> MELKHSISDYTEAEFLEFVKKICRAEGATEEDDNKLVREFERLTEHPDGSDLIYYPRDDREDSPEGIVKEIKEWRAANGKSGFKQGLEHHHHHH;> MESKRNKPGKATGKGKPVGDKWLDDAGKDSGAPIPDRIADKLRDKEFKNFDDFRKKFWEEVSKDPDLSKQFKGSNKTNIQKGKAPFARKKDQ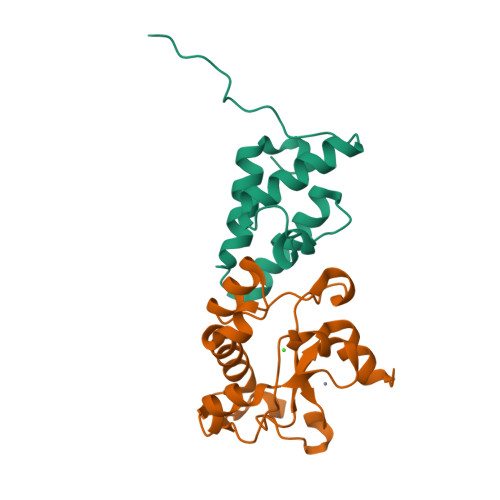VGGRERFELHHDKPISQDGGVYDMNNIRVTTPKRHIDIHRGK>[10x]MHADCAKGKIEFSKYNEDDTFTVKVDGKEYWTSRWNLQPLLQSAQLTGMT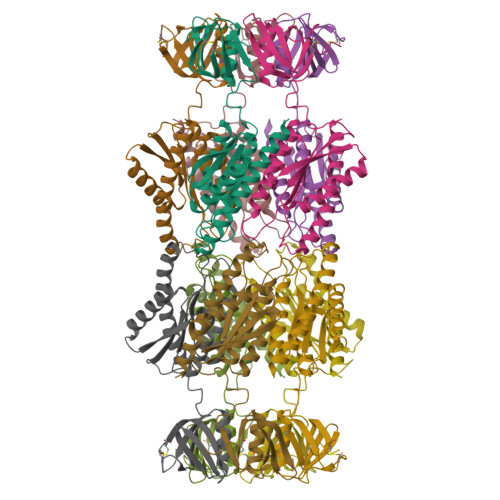VTIKSSTCESGSGFAEVQFNNDGSGSGSGSGSLKTSFKIAFIQARWHADIVDEARKSFVAELAAKTGGSVEVEIFDVPGAYEIPLHAKTLARTGRYAAIVGAAFVIDGGIYRHDFVATAVINGMMQVQLETEVPVLSVVLTPHHFHESKEHHDFFHAHFKVKGVEAAHAALQIVSERSRIAALV> MDRWNMHKPMLCDSLPTASRTAAAILNLAQREDVTAEALAQLIQTDPALTGRILRFANAPAQGTRRPVASVIDAIDLVGLPAVRQFALSLSLIDAHREGRCEAFDYAAYWQKSLARAVALQSITAQASTVAPKE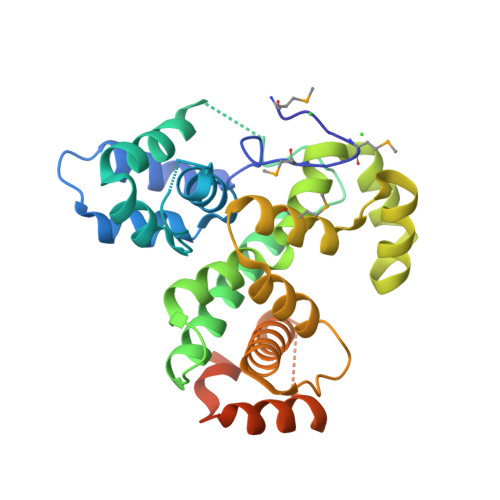AFTLGLLADVGRLALATAWPEEYSECLRKADGEALIALERERFATDHDELTRMLLTDWGFPQVFIDALQLSQQDEIRDEGRTGRFARQLALAQHIADHRLAEEPRRAALSPLLRAEARRCGLGDEDLARLLADPPADWLDWTRTIGLEHHHHHH>SASEEQVAQDTEEVFR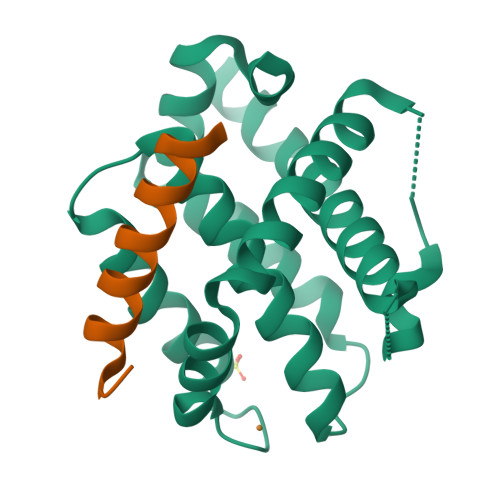SYVFYRHQQEQEAEGVAAPADPEMVTLPLQPSSTMGQVGRQLAIIGDDINRRYDSEFQTMLQHLQPTAENAYEYFTKIATSLFESGINWGRVVALLGFGYRLALHVYQHGLTGFLGQVTRFVVDFMLHHSIARWIAQRGGWVAALNLCNG[10x];>[10x]SSTMGQVGRQLAIIGDDINRRYGGC>[12x]MRSYDMNVETAAELSAVNDILASIGEPPVSTLEGDANADAANARRILNKINRQIQSRGWTFNIEEGITLLPDVYSNLIVYSDDYLSLMSTSGQSIYVNRGGYVYDRTSQSDRFDSGITVNIIRLRDYDEMPECFRYWIVTKASRQFNNRFFGAPEVEGVLQEEEDEARRLCMEYEMDYGGYNMLDGDAFTSGLLTR;>[18x]MANVIKTVLTYQLDGSNRDFNIPFEYLARKFVVVTLIGVDRKVLTINTDYRFATRTTISLTKAWGPADGYTTIELRRVTS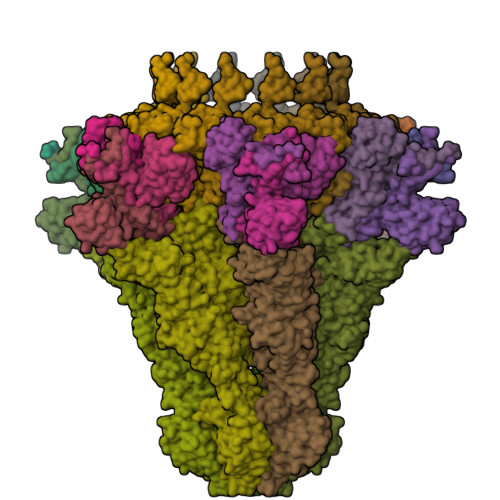TTDRLVDFTDGSILRAYDLNVAQIQTMHVAEEARDLTTDTIGVNNDGHLDARGRRIVNLANAVDDRDAVPFGQLKTMNQNSWQARNEALQFRNEAETFRNQAEGFKNESSTNATNTKQWRDETKGFRDEAKRFKNTAGQYATSAGNSASAAHQSEVNAENSATASANSAHLAEQQADRAEREADKLENYNGLAGAIDKVDGTNVYWKGNIHANGRLYMTTNGFDCGQYQQFFGGVTNRYSVMEWGDENGWLMYVQRREWTTAIGGNIQLVVNGQIITQGGAMTGQLKLQNGHVLQLESASDKAHYILSKDGNRNNWYIGRGSDNNNDCTFHSYVHGTTLTLKQDYAVVNKHFHVGQAVVATDGNIQGTKWGGKWLDAYLRDSFVAKSKAWTQVWSGSAGGGVSVTVSQDLRFRNIWIKCANNSWNFFRTGPDGIYFIASDGGWLRFQIHSNGLGFKNIADSRSVPNAIMVENE;>MALISQSIKNLKGGISQQPDILRYPDQGSRQVNGWSSETEGLQKRPPLVFLNTLGDNGALGQAPYIHLINRDEHEQYYAVFTGSGIRVFDLSGNEKQVRYPNGSNYIKTANPRNDLRMVTVADYTFIVNRNVVAQKNTKSVNLPNYNPNQDGLINVRGGQYGRELIVHINGKDVAKYKIPDGSQPEHVNNTDAQWLAEELAKQMRTNLSDWTVNVGQGFIHVTAPSGQQIDSFTTKDGYADQLINPVTHYAQSFSKLPPNAPNGYMVKIVGDASKSADQYYVRYDAERKVWTETLGWNTEDQVLWETMPHALVRAADGNFDFKWLEWSPKSCGDVDTNPWPSFVGSSINDVFFFRNRLGFLSGENIILSRTAKYFNFYPASIANLSDDDPIDVAVSTNRIAILKYAVPFSEELLIWSDEAQFVLTASGTLTSKSVELNLTTQFDVQDRARPFGIGRNVYFASPRSSFTSIHRYYAVQDVSSVKNAEDITSHVPNYIPNGVFSICGSGTENFCSVLSHGDPSKIFMYKFLYLNEELRQQSWSHWDFGENVQVLACQSISSDMYVILRNEFNTFLARISFTKNAIDLQGEPYRAFMDMKIRYTIPSGTYNDDTFTTSIHIPTIYGANFGRGKITVLEPDGKITVFEQPTAGWNSDPWLRLSGNLEGRMVYIGFNINFVYEFSKFLIKQTADDGSTSTEDIGRLQLRRAWVNYENSGTFDIYVENQSSNWKYTMAGARLGSNTLRAGRLNLGTGQYRFPVVGNAKFNTVYILSDETTPLNIIGCGWEGNYLRRSSGI[6x]3-methyl-2H-furo[2,3-c]pyran-2-one | C8 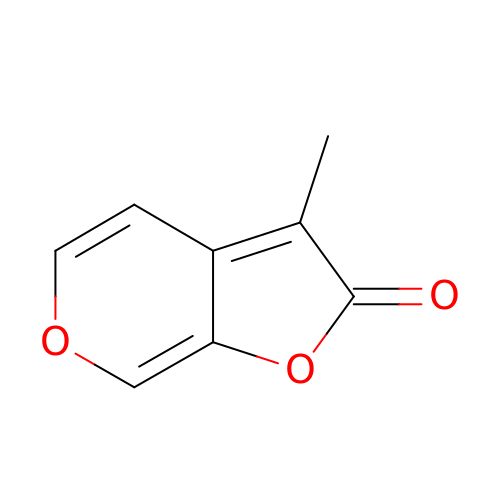H6 O3 | JUTMAMXOAOYKHT-UHFFFAOYSA-N> MFPKRILD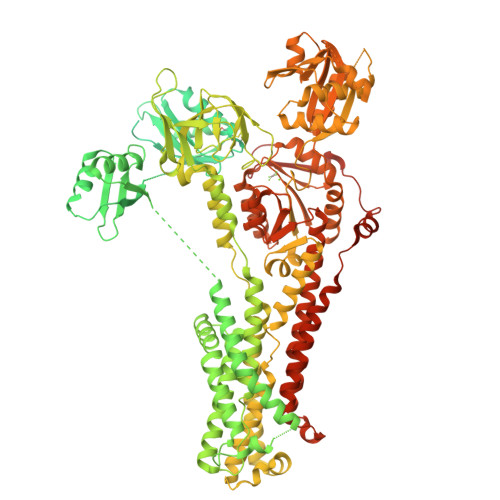EEEGVQLLSTENEKCSTKRRSSPQFCVNNTFSDSPVSVWKEAKKPSCAFDNRGYEGSPDDLCSLPDDVGSVVVAIQGMTCQSCVQSIEGRISKVSGVVGINVCLEQNNAIVNYLQTEITPHKICEEIEDMGFDASLSEQSGMPSSVKSSYYGDNVIKIRVEGMTCQSCVNTIEGKIGKIQGVQKIKVSLTGQEAVITYQSHIIQAEDLRKYIEDMGFEASIKNKPDPTKLGTIDIERLQNSIAENHSGHTNSNTVTLGIDGMHCKSCVHNIEGYVSGLAGIQSIRVSLKNKNAVVCLSQGSTSLLSLKESIENLPPGKFKVTLPVGVEKGQSLARNSTHSSHRDQSMGGNIAIISIGGMTCQSCVSSIENMISQRKGVLHILVSLDEGNGNIFYNPCETNAEELRAAIEDMGFHSTLVSDNSPSISCSEYNSKEEENKQTPPKATRQISGSRDYILDVLPKKSHPDFANEKYDTAPEKCFLQITGMTCISCVSNIERNLKKKDGIVSVLVALMSGKAEVKFYPDRIEPLEIAQLVEDLGFGASVMEDYTASDGNVELIITGMTCASCVHNIESRLMRTPGILQASVALATCKAQVKFDPEIVGPRDIIRIIEGIGFQASLAKRDPTAHKLDHKEEIKQWRNSFLFSLLFGIPVIILMIYMLAANKDHHNTMVLDRNIVPGLSIINLVFFILCTFVQTLGGRYFYVQAYKSLKHKATNMDVLIVLATTIAYIYSVVILTVAMVEKADKSPETFFDTPPMLFMFIALGRWLEHIAKSKTSEALAKLISLQATEAAVVTFGANQIILREEQVAVELVQRGDIVKVVPGGKFPVDGKVIEGTSMADESLITGEPMPVRKKPGSMVIAGSINAHGTVLVEATHVGSETTLAQIVKLVEEAQMSKAPIQQLADKISGYFVPFIIIISVVTLVTWIIIGFVNFDIIIKYFPSYSKNISKTEVIIRVAFQTSITVLSIACPCALGLATPTAVMVGTGVAAQNGILIKGGEPLEMAHKIKAVMFDKTGTITHGVPKVMRVLLLGDVVKMPLKRMLAVVGTAEASSEHPLGMAVTKYCKEELGTELLGYCTDFQAVPGCGISCKVNNIESVLVQNEEGLNEQNSYRNSLIGTTDSSLIITPELLGAQAPLAHTVLIGNREWMRRNGLHISTDVDEAMSSHEMKGQTAVLVAIDGELCGMIAIADTVKQEAALAVHTLKSMGIDVVLITGDNRKTAKAIATQVGIKKVFAEVLPSHKVAKVQALQSDNKRVAMVGDGVNDSPALARADVGIAIGTGTDVAIEAADIVLIRNDLLDVVASIHLSKRTVRRIRLNFVFALIYNLLGIPIAAGVFMPAGLVLQPWMGSAAMAASSVSVVLSSLQLKCYRKPDSDRYEARAQGHMKPLTPSQISVHIGMDDRWRDLPKTKAWDQISYISQVSRASQKPKRHGSLVEQQDKWSLLINETHEDQMI>MHHHHHHENLYFQSMSFPPQRYHYFLVLDFEATCDKPQIHPQEIIEFPILKLNGRTMEIESTFHMYVQPVVHPQLTPFCTELTGIIQAMVDGQPSLQQVLERVDEWMAKEGLLDPNVKSIFVTCGDWDLKVMLPGQCQYLGLPVADYFKQWINLKKAYSFAMGCWPKNGLLDMNKGLSL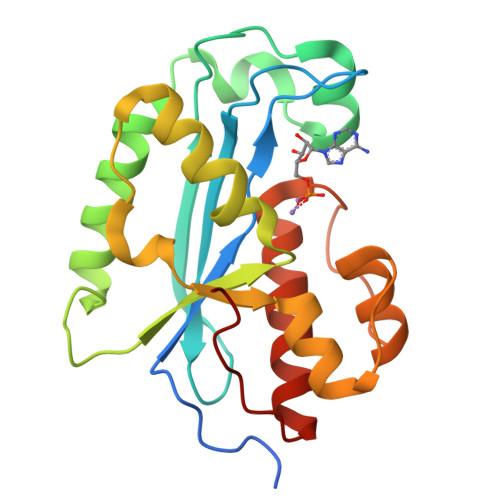QHIGRPHSGIDDCKNIANIMKTLAYRGFIFKQTSKPF[2x]cyanidin | C15 H11 O6 | 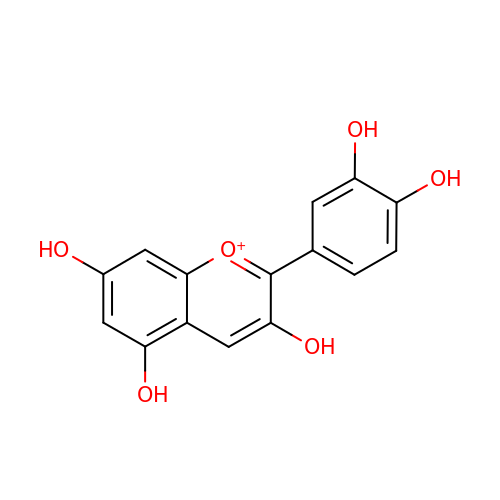VEVZSMAEJFVWIL-UHFFFAOYSA-O>[2x]MARQLRAEQTRATIIGAAADLFDRRGYESTTLSEIVAHAGVTKGALYFHFAAKEDLAHAILEIQSRTSRRLAKDLDGRGYSSLEALMRLTFGMA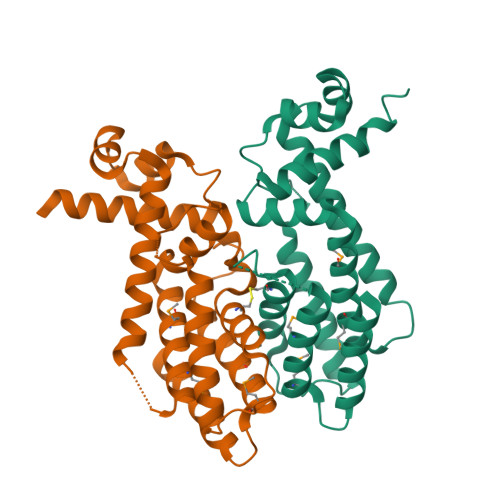RLCVQGPVLRAGLRLATAGVPVRPPLPHPFTEWREIATSRLLDAVRQSDVHQDIDVDSVAHTLVCSVVGTRVVGGTLEPAGREPRRLAEMWYILIRGMVPVTRRARYVTLAARLEQETGTA> PISPIETVPVKLKPGMDGPKVKQWPLTEEKIKALVEICTEMEKEGKISKIGPENPYNTPVFAIKKKDSTKWRKLVDFRELNKRTQDFWEVQLGIPHPAGLKKKKSVTVLDVGDAYFSVPLDEDFRKYTAFTIPSINNETPGIRYQYNVLPQGWKGSPAIFQSSMTKILEPFRKQNPDIVIYQYMDDLYVGSDLEIGQHRTKIEELRQHLLRWGLYTPDKKHQKEPPFLWMGYELHPDKWTVQPIVLPEKDSWTVNDIQKLVGKLNWASQIYPGIKVRQLCKLLRGTKALTEVIPLTEEAELELAENR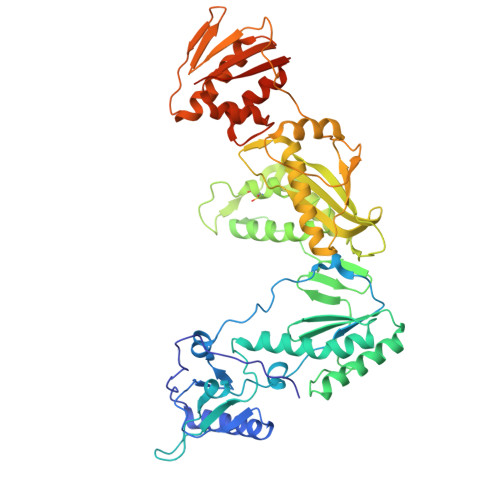EILKEPVHGVYYDPSKDLIAEIQKQGQGQWTYQIYQEPFKNLKTGKYARMRGAHTNDVKQLTEAVQKITTESIVIWGKTPKFKLPIQKETWETWWTEYWQATWIPEWEFVNTPPLVKLWYQLEKEPIVGAETFYVDGAANRETKLGKAGYVTNRGRQKVVTLTDTTNQKTELQAIYLALQDSGLEVNIVTDSQYALGIIQAQPDQSESELVNQIIEQLIKKEKVYLAWVPAHKGIGGNEQVDKLVSAGIRKVL> HHHHHHMASSAQDGNNPLFSPYKMGKFNLSHRVVLAPMTRCRALNNIPQAALGEYYEQRATAGGFLITEGTMISPTSAGFPHVPGIFTKEQVREWKKIVDVVHAKGAVIFCQLWHVGRASHEVYQPAGAAPISSTEKPISNRWRILMPDGTHGIYPKPRAIGTYEISQVVEDYRRSALNAIEAGFDGIEIHGAHGYLIDQFLKDGINDRTDEYGGSLANRCKFITQVVQAVVSAIGADRVGVRVSPAIDHLDAMDSNPLSLGLAVVERLNKIQLHSGSKLAYLHVTQPEYVAYGQTEAGRLGSEEEEARLMRTLRNAYQGTFICSGGYTRELGIEAVAQGDADLVSYGRLFISNPDLVMRIKLNAPLNKYNRKTFYTQDPVVGYTDYPFLQGNGSNGPLSRL

Jasmonates are phytohormones that are pivotal in mediating plant responses to various biotic and abiotic stresses and regulating plant growth. The first crystal structure of OPR3 from tomato (SlOPR3) showed that the enzyme crystallized as a self-inhibitory dimer in which the L6 loop, a critical loop involved in substrate recognition and coenzyme binding, from each protomer intrudes into the active site cavity of the other protomer. Based on these observations, it was postulated that the formation of the self-inhibitory homodimer represents a mechanism for regulating OPR3 activity and, thereby, jasmonic acid biosynthesis.

The crystal structure of R283E is almost identical to that of the wild type (RMSCα = 0.22 Å), except for the R283E substitution and L6, which lacks 16 amino acids (V285–E301) due to disorder. As R283E initially failed to form a homodimer in crystallo, we assumed that the amino acid exchange disrupted dimer-forming and -stabilizing interactions. However, our DLS results showed that at higher concentrations, the monomer–dimer equilibrium is clearly shifted toward the dimer. R283E showed the strongest tendency toward the monomeric state among the variants, as even at a concentration of 5 mg/ml, it exhibited mainly the monomeric state. Structurally, it is unclear why R283E prefers to crystallize in its monomeric form while R283D prefers the dimeric form. Considering both the DLS and crystallographic data, it seems that the amino acid substitution R283E increases the flexibility of loop L6 in the corresponding variant, impeding proper dimer formation.> TPAFNKPKVELHVHLDGAIKPETILYFGKKRGIALPADTVEELRNIIGMDKPLSLPGFLAKFDYYMPVIAGCREAIKRIAYEFVEMKAKEGVVYVEVRYSPHLLANSKVDPMPWNQTEGDVTPDDVVDLVNQGLQEGEQAFGIKVRSILCCMRHQPSWSLEVLELCKKYNQKTVVAMDLAGDETIEG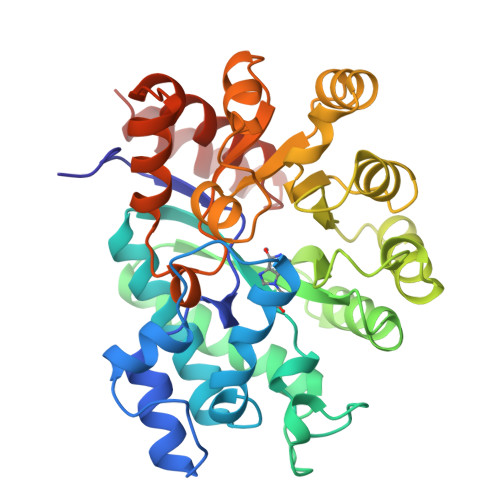SSLFPGHVEAYEGAVKNGIHRTVHAGEVGSPEVVREAVDILKTERVGAGYHTIEDEALYNRLLKENMHFEVCPWSSYLTGAWDPKTTHAVVRFKNDKANYSLNTDDPLIFKSTLDTDYQMTKKDMGFTEEEFKRLNINAAKSSFLPEEEKKELLERLYREYQ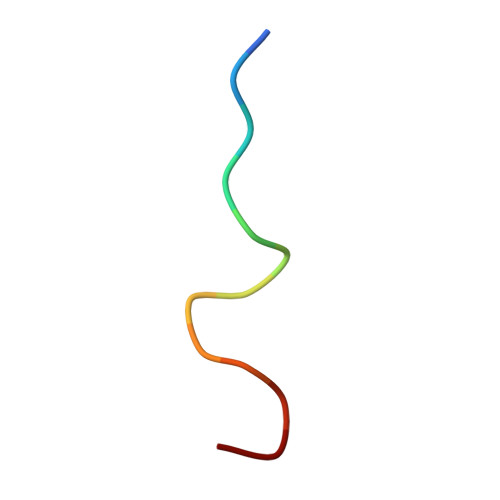> QAQGPPYPTYPGY Proliferating cell nuclear antigen (PCNA) is an essential cofactor for DNA replication and repair, recruiting multiple proteins to their sites of action. The proliferating cell nuclear antigen (PCNA) has a central role during DNA replication, acting to recruit enzymes to the DNA replication fork, and to modify enzymatic activity and processivity. PCNA also regulates entry into S-phase via interactions with the cell cycle regulator p21 and the pre-replication complex component Cdt1. These PCNA partners all utilise a similar peptide motif to associate with PCNA, the PCNA-interacting-protein (PIP) box.

We examined the effects of the PCNAS228I mutation that causes PCNA-associated DNA repair disorder (PARD). Diffraction quality crystals in P43212 space group grew after 10 days at 20 °C, set up in a 1:1 protein:precipitant volume ratio with well buffer containing 2 M (NH4)2SO4 and 0.1 M NaOAc pH 4.5. Data up to 2.27 Å was collected on the i03 beamline at the Diamond Light Source, Didcot, UK. The overall structure of PCNA is retained by PCNAS228I, it is a recognisable toroidal trimer, with pseudo-6 fold symmetry and a central hole through which double-stranded DNA will fit. There is no evidence of trimer destabilisation, as the monomer–monomer interface appears unperturbed when compared to published structures of PCNAWT. The structure is of sufficient resolution that the electron density of the isoleucine substitution can be identified. The larger isoleucine side chain has a steric clash with Tyr133 in the standard position, forcing a 90° rotation of the sidechain of Tyr133, which in turn repositions a significant proportion of the IDCL (amino acids Gly127 to Asp120). The S228I change has very little effect on the overall structure and whilst the total rmsd between our S228I structure and wild type structure is 0.6 Å, the local rmsd averaged over the three IDCL regions (residues 120–130) is 1.9 Å. Many of the residues of PCNA that are most affected by the S228I change coincide with those IDCL residues sitting at the interface between PCNA and PIP box containing proteins, such as p21 and Fen1. It thus appears that this dramatic structural reorganisation of the IDCL, resulting from the single amino acid change in the PCNAS228I protein is likely to prevent this binding surface from operating correctly.

>MFEARLVQGSILKKVLEALKDLINEACWDISSSGVNLQSMDSSHVSLVQLTLRSEGFDTYRCDRNLAMGVNLTSMSKILKCAGNEDIITLRAEDNADTLALVFEAPNQEKVSDYEMKLMDLDVEQLGIPEQEYSCVVKMPSGEFARICRDLSHIGDAVVISCAKDGVKFSASGELGNGNIKLSQTSNVDKEEEAVTIEMNEPVQLTFALRYLNFFTKATPLSSTVTLIMSADVPLVVEYKIADMGHLKYYLAPKIEDE[3x]>[4x]STFSKAAPSVPSKPSDCNFISNFYSHSRLHHISMWKCELTEFVNTLQRQSNGIFPGREKLKKMKTGRSALVVTDTGDMSVLNSPRHQSCIMHVDMDCFFVSVGIRNRPDLKGKPVAVTSNRGTGRAPLRPGANPQLEWQYYQNKILKGKAADIPDSSLWENPDSAQANGIDSVLSRAEIASCSYEARQLGIKNGMFFGHAKQLCPNLQAVPYDFHAYKEVAQTLYET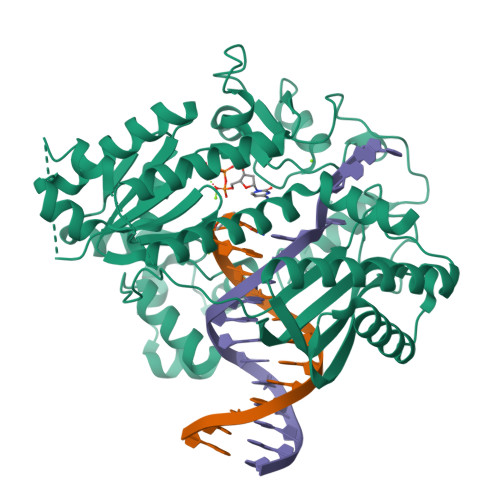LASYTHNIEAVSCDEALVDITEILAETKLTPDEFANAVRMEIKDQTKCAASVGIGSNILLARMATRKAKPDGQYHLKPEEVDDFIRGQLVTNLPGVGHSMESKLASLGIKTCGDLQYMTMAKLQKEFGPKTGQMLYRFCRGLDDRPVRTEKERKSVSAEINYGIRFTQPKEAEAFLLSLSEEIQRRLEATGMKGKRLTLKIMVRKPGAPVETAKFGGHGICDNIARTVTLDQATDNAKIIGKAMLNMFHTMKLNISDMRGVGIHVNQLVPTNLNPST> MGRIEVVNVSHIFHRGTPLEKKALENVSLVINEGECLLVAGNTGSGKSTLLQIVAGLIEPTSGDV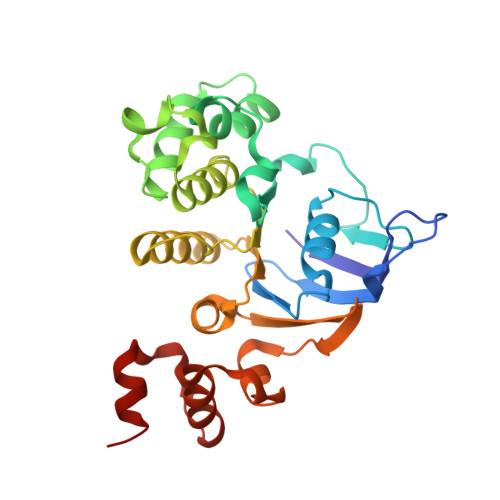LYDGERKKGYEIRRNIGIAFQYPEDQFFAERVFDEVAFAVKNFYPDRDPVPLVKKAMEFVGLDFDSFKDRVPFFLSGGEKRRVAIASVIVHEPDILILDEPLVGLDREGKTDLLRIVEKWKTLGKTVILISHDIETVINHVDRVVVLEKGKKVFDGTRMEFLEKYDPRFFTSKMLVMRRLVLKGEDPFSMSDDELLERVCNS>MSQHNEKNPHQHQSPLHDSSEAKPGMDSLAPEDGSHRP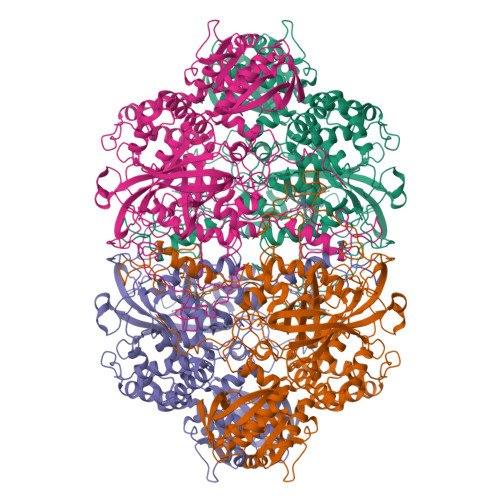AAEPTPPGAQPTAPGSLKAPDTRNEKLNSLEDVRKGSENYALTTNQGVRIADDQNSLRAGSRGPTLLEDFILREKITHFDHERIPERIVHARGSAAHGYFQPYKSLSDITKADFLSDPNKITPVFVRFSTCQGGAGSADTVRDIRGFATKFYTEEGIFDLVGNNTPIFFIQDAHKFPDFVHAVKPEPHWAIPQGQSAHDTFWDYVSLQPETLHNVMWAMSDRGIPRSYRTMEGFGIHTFRLINAEGKATFVRFHWKPLAGKASLVWDEAQKLTGRDPDFHRRELWEAIEAGDFPEYELGFQLIPEEDEFKFDFDLLDPTKLIPEELVPVQRVGKMVLNRNPDNFFAENEQAAFHPGHIVPGLDFTNDPLLQGRLFSYTDTQISRLGGPNFHEIPINRPTCPYHNFQRDGMHRMGIDTNPANYEPNSINDNWPRETPPGPKRGGFESYQERVEGNKVRERSPSFGEYYSHPRLFWLSQTPFEQRHIVDGFSFELSKVVRPYIRERVVDQLAHIDLTLAQAVAKNLGIELTDDQLNITPPPDVNGLKKDPSLSLYAIPDGDVKGRVVAILLNDEVRSADLLAILKALKAKGVHAKLLYSRMGEVTADDGTVLPIAATFAGAPSLTVDAVIVPCGNIADIADNGDANYYLMEAYKHLKPIALAGDARKFKATIKIADQGEEGIVEADSADGSFMDELLTLMAAHRVWSRIPKIDKIPA[4x]> GSLLDEIMAQTRIAPSEEGYDIAKKGVAAFIENLMGSQHSAEPVNKSLVDQMLVELDKKISAQMDEILHNSQFQAMESAWRGLKLFVDRTDFRENNKVEILHVTKDELLEDFEFAPETAQSGLYKHVYSAGYGQFGGEPVGAIIGNYAFTPSTPDMKLLQYMGALGAMAHAPFISSVGPEFFGIDSFEELPNIKDLKSTFESPKYTKWRSLRESEDARYLGLTAPRFLLRVPYDPIENPVKSFNYAENVSASHEHYLWGNTAFAFATRLTDSFAKYRWCPNIIGPQSGGAVEDLPVHVFESMGALQSKIPTEVLITDRKEFELAEEGFIALT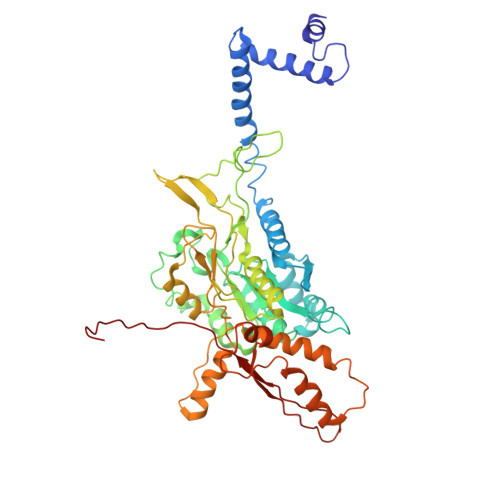MRKGSDNAAFFSANSIQKPKVFPNTKEGKEAETNYKLGTQLPYMMIINRLAHYVKVLQREQIGAWKERQDLERELNSWIKQYVADQENPPADVRSRRPLRAARIEVMDVEGNPGWYQVSLSVRPHFKYMGANFELSLVGRL> MLEEIMKYEASILTHDSSIRYLQEIYNSNNQKIVNLKEKVAQLEAQCQEPCKDTVQIHDITGKDCQDIANKGAKQSGLYFIKPLKANQQFLVYCEIDGSGNGWTVFQKRLDGSVDFKKNWIQYKEGFGHLSPTGTTEFWLGNEKIHLISTQSAIPYALRVELEDWNGRTSTADYAMFKVGPEADKYRLTYAYFAGGDAGDAFDGFDFGDDPSDKFFTSHNGMQFSTWDNDNDKFEGNCAEQDGSGWWMNKCHAGHLNGVYYQGGTYSKASTPNGYDNGIIWATWKTRWYSMKKTTM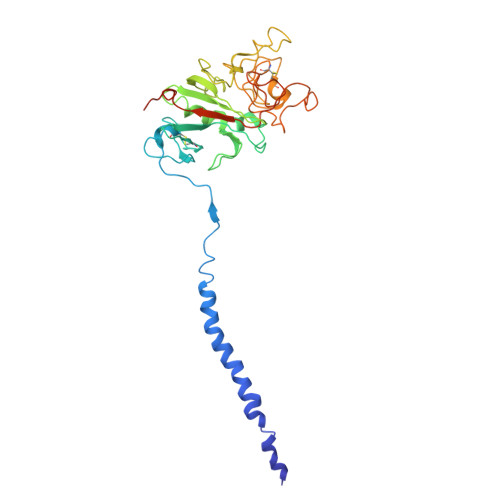KIIPFNRLTIGEGQQHHLGGAKQAGDV>[6x]HMKIAIFGTVGAGKSTISAEISKK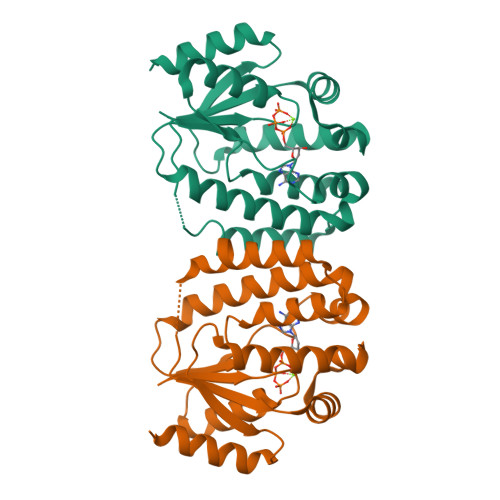LGYEIFKEPVEENPYFEQYYKDLKKTVFKMQIYMLTARSKQLKQAKNLENIIFDRTLLEDPIFMKVNYDLNNVDQTDYNTYIDFYNNVVLENLKIPENKLSFDIVIYLRVSTKTAISRIKKRGRSEELLIGEEYWETLNKNYEEFYKQNVYDFPFFVVDAELDVKTQIELIMNKLNSIKNPN>MDHRRLGV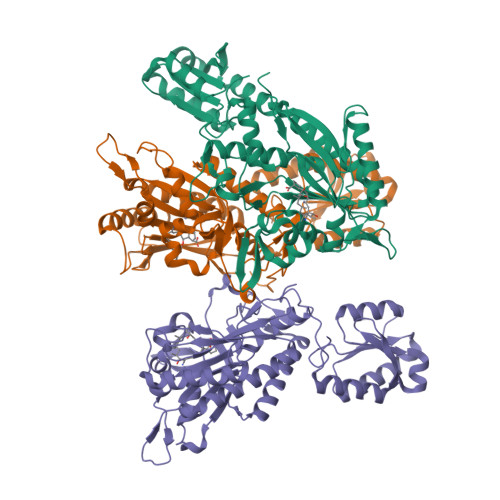SEELFFFHSLSPGSGFWLPHGSAIYFKLLKFIREQYRARGYTEVITPNIFNMELWNISGHAKHYKENMFVFDVEGQEYALKPMNCPAASLMFDFRQRSYRELPIRYADCGVLHRNELSGALTGLTRVRRFQQDDAHIFCRDDQIKKEVLDFLSFMKYVYDVFGIEFNLELSTRPEKAMGELEQWERAESQLAEALDEFVGAGKWVVNPGDGAFYGPKIDIMITDALKRQHQCATVQLDFQLPIRFNLKYRTDDADNFKRPVIIHRAIYGSLERFVAVLVEHYAGKFPFWLSPRQVLIVTVGAAFVDYGYEVKDAMFRAGFDVDIDDTGKTLNKKIREGQMAHYNFILVVGAHEKETRSVNIRTRDNKVTGTKTLEEAIAMFKELEETKAADEHHHHHH[3x]>AECSVDIQGND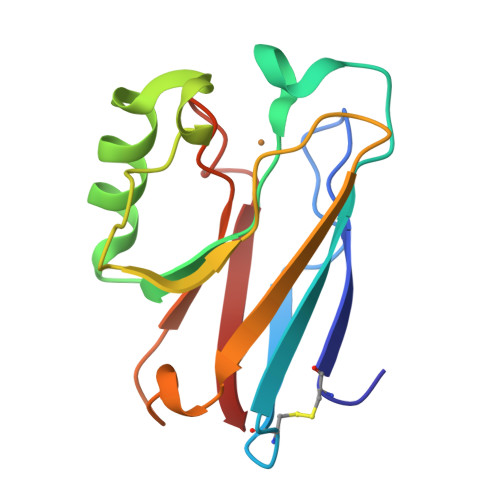QMQFNTNAITVDKSCKQFTVNLSHPGNLPKNVMGHSWVLSTAADMQGVVTDGMASGLDKDYLKPDDSRVIAHTKLIGSGEKDSVTFDVSKLKEGEQYMFFCTFPGHSALLKGTLTLK[2x]>MSTIKPVSVKLDADIKARVEHLAETRKRSSHWMMREAIREYVEREEKREALQQEALRAWEEHQTSGLHVTGDEVVSWLESWGSENEQAALHATNSLHCHCIT[2x];>[2x]MPQIVFT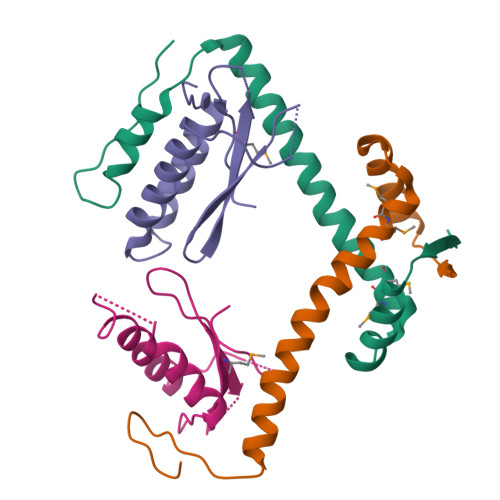ATALRDLERLREFLRSKNPPAAQRAASAIINTIRKLESYPDIGRPIDDNDFSFRELLIDFGDTGYLAMYQYDGGERLTVLCIRHQKEAGY>MELCSGKPFDAFTDLKNGSLFAFRGQYSYELDEKAVRPGYPKLIRDVWGIEGPIDAAFTRINSQGKTYLFKGSQYWRFEDGVLDPDYPRNISDGFDGIPDNVDAALALPAHSYSGRERVYFFKGKQYWEYQFQRTSAGTRQPQFISRDWHGVPGQVDAAMAGRISVFFFSGDKYYRVNLRTRRVDTVDPPYPRSIAQYWLG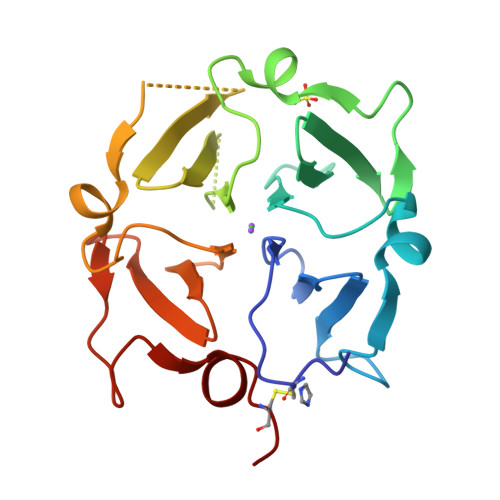CPA[2x]> GLTIDLKNFRKPGEKTFTQR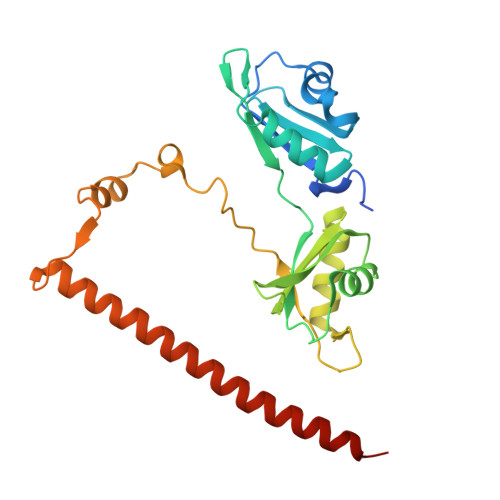SRLFVGNLPPDITEEEMRKLFEKYGKAGEVFIHKDKGFGFIRLETRTLAEIAKVELDNMPLRGKQLRVRFACHSASLTVRNLPQYVSNELLEEAFSVFGQVERAVVIVDDRGRPSGKGIVEFSGKPAARKALDRCSEGSFLLTTFPRPVTVEPMDQLDDEEGLPEKLVIKNQQFHKEREQPPRFAQPGSFEYEYAMRWKALIEMEKQQQDQVDRNIKEAREKLEMEMEAARHEHQVMLM>MAVNVYSTSV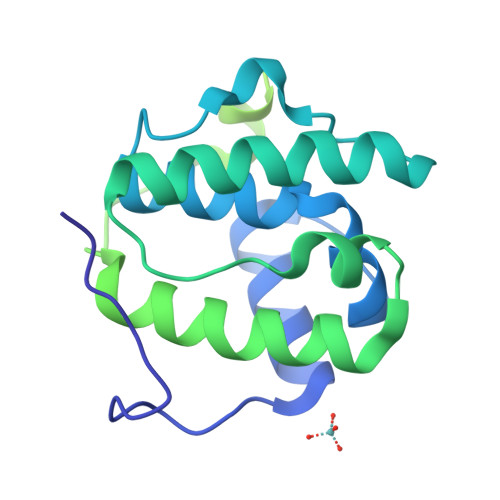TSDNLSRHDMLAWINESLQLNLTKIEQLCSGAAYCQFMDMLFPGSIALKKVKFQAKLEHEYIQNFKILQAGFKRMGVDKIIPVDKLVKGKFQDNFEFVQWFKKFFDANYDGKDYDPVAARQGQETAVAPSLVAPALNKPKKPLTSSSAAPQRPISTQRTAAAPKAGPGVVRKNPGVGNGDDEAAELMQQVNVLKLTVEDLEKERDFYFGKLRNIELICQENEGENDPVLQRIVDILYATDEGFVIPDEGGPQEEQEEY[2x]>[3x]SSGMQIGKIIKVSGPLVMAENMSEASIQDMCLVGDLGVIGEIIEMRQDVASIQVYEETSGIGPGEPVRSTGEALSVELGPGIISQMFDGIQRPLDTFMEVTQSNFLGRGVQLPALDHEKQWWFEATIEEGTEVSAGDIIGYVDETKIIQHKIMVPNGIKGTVQKIESGSFTIDDPICVIETEQGLKELTMMQKWPVRRGRPIKQKLNPDVPMITGQRVIDTFFPVTKGGAAAVPGPFGAGKTVVQHQIAKWSDVDLVVYVGCGERGNEMTDVVNEFPELIDPNTGESLMERTVLIANTSNMPVAAREASIYTGITIAEYFRDMGYDVAIMADSTSRWAEALREMSGRLEEMPGDEGYPAYLGSRLAEYYERSGRVIALGSDQREGSITAISAVSPSGGDISEPVTQNTLRVVKVFWGLDSSLAQKRHFPSINWIQSYSLYSTEVGRYMDQILQQDWSDMVTEGMRILQEEEQLNEIVRLVGIDSLSDNDRLTLEVAKSIREDYLQQNAFDDVDTFTSREKQFNMLKVILTFGKEARKALSLGAYFNEIMEGTVAVRERISRSKYIPEEELAKISSINEEIKETIQLIVSEGGM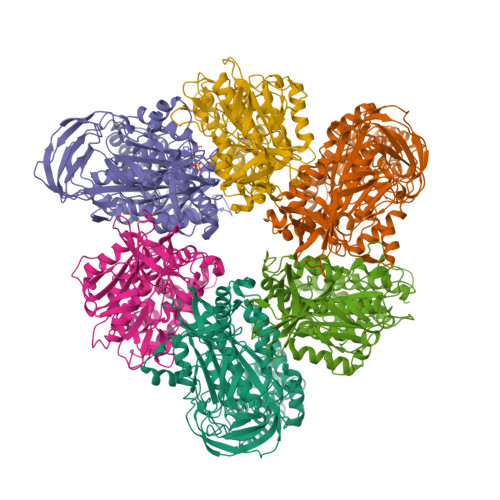TDD;>[3x]MIKEYRTIKEVVGPLMAVEKVSGVKYEELIEVRMQNGEIRRGQVLEVQEDKAMVQIFEGTSGINLKNSSVRFLGHPLQLGVSEDMIGRVFDGLGRPKDNGPEILPEKYLDINGEVINPIARDYPDEFIQTGISAIDHLNTLVRGQKLPVFGPPGAGKSALAAQIARQATVLDSSDDFAVVFAAIGITFEEAEFFMEDFRQTGAIDRSVMFMNLANDPAIERIATPRMALTAAEYLAYEKGMHVLVIMEDMTNYAEALREISAARREVPGRRGYPGYLYTNLATLFERAGRIRGLKGSVTQIPILTMPEDDKTHPIPDLTGYITEGQIILTRELYKSGISPPIDVLPSLSRLKDKGTGAGKTREDHAATMNQLFAAYAQGKQAKELAVVLGESALSDIDKIYAKFAERFENEYVNQGFYTNRTITETLDLGWELLAMLPRTELKRIKDDLLDKYLPEGK> EMETYVNKLHEGSTYTAAVQYNVLEKDDDPASLTIWVPM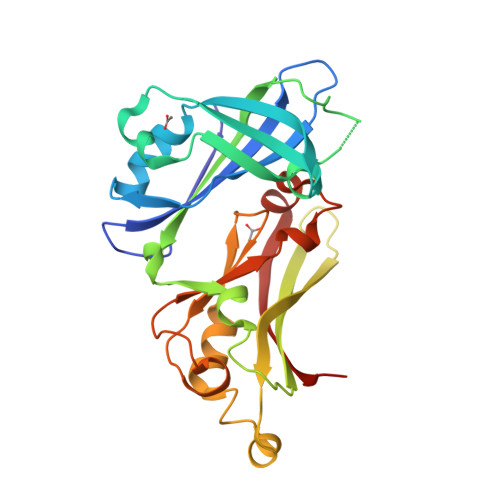FQSSMPADLLIKELANVNILVKQISTPKGPSLRVMINSRSAVLAQMPSKFTICANVSLDDRSKLAYDVTTPCEIKACSLTCLKSKNMLTTVKDLTMKTLNPTHDIIALCEFENIVTSKKVIIPTYLRSISVRNKDLNTLENITTTEFKNAITNAKIIPYSGLLLVITVTDNKGAFKYIKPQSQFIVDLGAYLEKESIYYVTTNWKHTATRFAIKPMED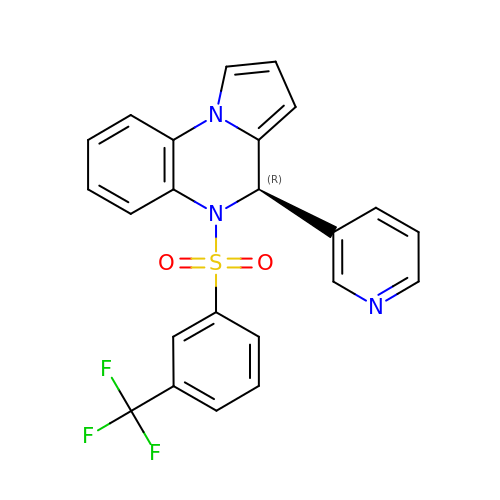(4~{R})-4-pyridin-3-yl-5-[3-(trifluoromethyl)phenyl]sulfonyl-4~{H}-pyrrolo[1,2-a]quinoxaline | C23 H16 F3 N3 O2 S | UAZQZAONUXSURN-JOCHJYFZSA-N> RRSTESEKAPSETEISQIVEWIEQRYQQTKAHQTLAAWEYGSNLTEFNLSKKTKAAADFAEVAKAVAEELQQFKTDQLTNATLKRRIKKLAKLGYAALPADQFKELLGAIASMESNYAKAKFCAYGDATKCDLSLDPELTEIFANHREPEELKYYWVQWYNATGAPVRESFQKYVELNRQAALRNNFSSGAAVWLNEYDDSTFEQ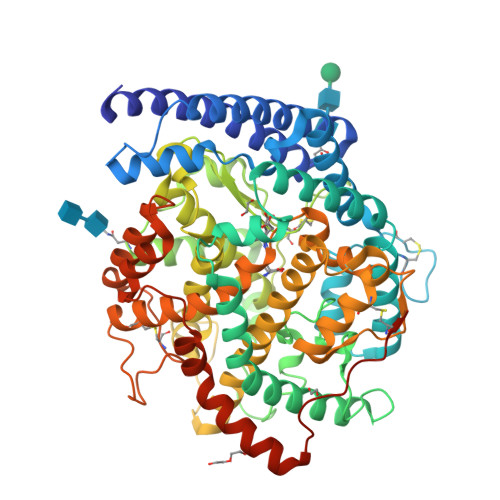QVDDVIEQIRPLYEQLHAYVRYKLRQKYGDKLVSPTGPIPMHLLGNLWAQTWDNIADFTTPFPEKKLLDVTDEMIRQGYTPIKMFQMGDDFFTSLNMTKLPQTFWDKSILEKPTDGRDLVCHASAWDFFAIDDVRIKQCTRVNMREFFVVHHELGHIQYYLQYQHQPVEFRGGANPGFHEAVGDVLSLSVSTPKHLKKVGLLKDYEEDEQVKINQFYRAGVTKLVFLPFAYTLDKYRWGVFRGDIKPREYNCKFWEMRSRYSGVEPPVVRTEQDFDPPAKYHVSADVEYLRYFVSYVIQFQFHRAACALAGEYVKGDPEKTLNNCDIYQSTAAGNQLKEMLALGSSKPWPDAMEVLTGERKMSADAILEYFDPLYQWLLEENKRLGAHVGWTDSQKCVSHPIDFMAAKHHHHHHHH>GPGSMIQTVVKRDGRIVGFNEQKIMAAIRKAMLHTDKGEDTTLIEQITDHISYRGKSQMSVEAIQDAIEMELMKSARKDVAQKYIAYRNQRNIARKAKTRDVFMSIVNAKNNDITRENANMNADTPAGMMMKFASETTKPFVDDYLLSEDVRDAVMHNYIHIHDKDYYPTKSLTCVQHPLDVILNHGFTAGHGSSRPAKRIETAAVLACISLETCQNEMHGGQAIPAFDFYLAPYVRMSYQEEVKNLEKLTGEDLSNLYDAPIDDYIEKPLDGLQGRERLEQHAINKTVNRVHQAMEAFIHNMNTIHSRGGNQVVFSSINYGTDTSAEGRCIMREILQSTYQGVGNGETAIFPIQIWKKKRGVNYLPEDRNYDLYKLACKVTARRFFPNFLNLDATFNQNEKWRADDPERYKWEIATMGCRTRVFEDRWGEKTSIARGNLSFSTINIVKLAIECMGIENEKQRIDMFFAKLDNILDITAKQLDERFQFQKTAMAKQFPLLMKYLWVGAENLKPEETIESVINHGTLGIGFIGLAECLVALIGKHHGESEKAQELGLKIITYMRDRANEFSEQYHHNYSILATPAEGLSGKFTKKDRKQFGVIPGVTDRDYYTNSNHVPVYYKCTALKKAQIEAPYHDLTRGGHIFYVEIDGDATHNPSVIESVVDMMDKYNMGYGSVNHNRNRCLDCGYENADAHLEVCPKCGSHHIDKLQRITGYLVGTTDRWNSGKLAELHDRVTHIGGEK[4x]

RNRs produce all four deoxyribonucleotides and are the only enzymes providing de novo building blocks for DNA replication and repair in all free-living organisms. Class III RNRs, which only function anaerobically, are dimers of an α subunit (NrdD) with a stable radical close to the active site, and binding sites for allosteric nucleotides. Binding of ATP activates RNR, and binding of dATP inhibits it. Here, we present structural, biochemical, and biophysical studies on the ATP-cone-containing NrdD from the human pathogen Prevotella copri (PcNrdD; Nii et al., 2023), showing that the binding of dATP causes increased flexibility of the C-terminal glycyl radical-bearing domain, as well as a flap-like loop that binds across the top of the active site in the active form.

From the same micrographs that revealed the dATP-bound dimers we also resolved dATP-bound tetramers. We obtained a map from cryoSPARC at 2.8 Å, which was again improved with DeepEMhancer. Two dATP molecules are bound to each ATP-cone and one at each of the specificity sites, giving a total of 12 visible dATPs per tetramer. The tetramer reveals an arrangement of two dimers (chains A/B and C/D, respectively) in which the ATP-cones are all well-ordered and one ATP-cone from each pair mediates interactions between the dimers. The ATP-cones have an almost domain-swapped arrangement within each dimer relative to the core domains. Remarkably, the pair of ATP-cones is highly asymmetrically positioned with respect to the twofold axis of its core dimer, being displaced as a rigid body towards the other dimer. The asymmetric arrangement is associated with two distinct conformations of the linker 93–103 between the fourth helix of the ATP-cone and the core domain. The rest of the polypeptide between residues 103 and 121, including the NxN flap, is disordered in both linkers. Interestingly, all contacts between the two dimers of the tetramer are mediated by interactions between one of the ATP-cones in one dimer (B or D) and one of the core domains of the other dimer (C or A, respectively). The amount of buried surface area is small: 717 Å2, or around 1% of the total surface area of each dimer.>YVSESEPLVRFKNSVKITKGDLNSWREGTDPCSGKWFGIYCQKGLTVSGIHVTRLGLSGTITVDDLKDLPNLKTIRLDNNLLSGPLPHFFKLRGLKSLMLSNNSFSGEIRDDFFKDMSKLKRLFLDHNKFEGSIPSSITQLPQLEELHMQSNNLTGEIPPEFGSMKNLKVLDLSTNSLDGIVPQSIADKKNLAVNLTENEYLCGPVVDVGCENIELNDPQEGQPPSKPSSSVPETSHHHHHH[2x];> TLINGSSDEERTYSFSPTTSPFDPRSLNQELKIGRIGYCFDCARACMRRGKYIRTCSFERKLCRCSISDIK

Orthologs of LURE1 in Torenia concolor (TcCRP1)15 and A. thaliana (AtLURE1)9 were recently shown as key attractant molecules, indicating a significant role played by these secreted proteins in pollen tube guidance. By contrast, our data showed that the LRR-RK PRK6 expressed at the tip of pollen tube is an essential receptor of the same attractant peptide and important for targeting of pollen tube to ovule in the pistil. In the current study, we present biochemical, structural and functional evidence showing that AtPRK6 functioned as a receptor of AtLURE1, strongly supporting previous genetic data. Sharply contrasting with other LRR-RKs, AtPRK6 recognizes AtLURE1.2 through the C-terminal loop of its LRR domain rather than the LRR portion.

In order to probe the recognition mechanism of AtLURE1 peptides by AtPRK6 at atomic level, we solved the crystal structures of the AtLURE1.2-AtPRK6LRR complex crystallized in two different forms by molecular replacement. The AtLURE1.2-AtPRK6LRR protein complexes in the two crystal forms display a nearly identical structure. Two AtPRK6LRR molecules exist in one asymmetric unit of the crystal with higher resolution. Interestingly, one of the molecules is in an AtLURE1.2-free state. The C-terminal loop of the apo-AtPRK6LRR including Cys237 and Cys229, is disordered. In contrast, these two cysteine residues in AtLURE1.2 bound AtPRK6LRR form a disulfide bond that is involved in interaction with AtLURE1.2. These structural observations suggest that the disulfide bond-stabilized C-terminal loop is likely important for AtPRK6 LRR interaction with AtLURE1.2 in vitro. The C-terminal loop of AtPRK6LRR is mainly responsible for its interaction with AtLURE1.2. Arg83 of AtLURE1.2 is located at the center of the AtLURE1.2-AtPRK6LRR interface by being sandwiched between the C-terminal loop and C-terminal extension of the last LRR of AtPRK6LRR, forming hydrogen bonds with the carboxyl oxygen atoms of Tyr227 and Cys237 of AtPRK6LRR. Additionally, this arginine residue tightly stacks against the disulfide bond formed between Cys229 and Cys237 of AtPRK6LRR.> MLQYPELPLESPLIDAELPDPRGGRYRLSQFHEPLLAVVFMCNHCPYVKGSIGELVALAERYRGKVAFVGINANDYEKYPEDAPEKMAAFAEEHGIFF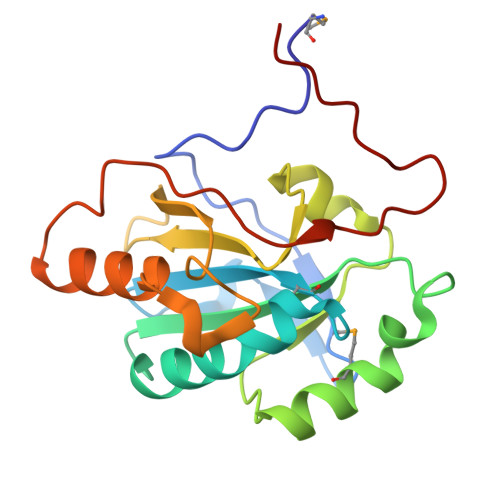PYLLDETQEVAKAYRALRTPEVFLFDERRLLRYHGRVNDNPKDPSKVQSHDLEAAIEALLRGEEPPLKEAPAIGCTIKWRPGNEPEVRIG>MGHHHHHHMLHLLEQIRAYCETCWEWQEAHEPGMDQDKNPMPAPVEHQICPAVCVLMKLSFDEEHRHAMNELGGLQAIAELLQVDCEMYGLTNDHYSITLRRYAGMALTNLTFGDVANKATLCSMKGCMRALVAQLKSESEDLQQVIASVLRNLSWRADVNSKKT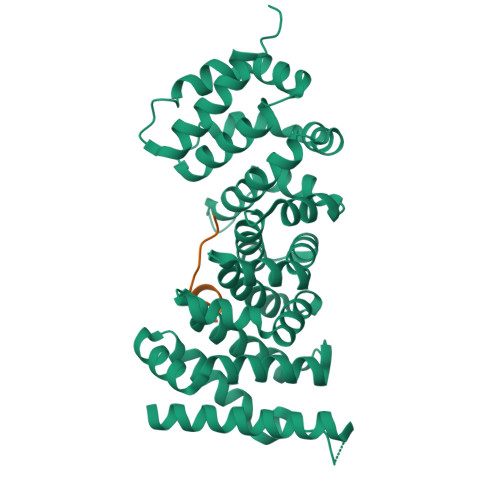LREVGSVKALMECALEVKKESTLKSVLSALWNLSAHCTENKADICAVDGALAFLVGTLTYRSQTNTLAIIESGGGILRNVSSLIATNEDHRQILRENNCLQTLLQHLKSHSLTIVSNACGTLWNLSARNPKDQEALWDMGAVSMLKNLIHSKHKMIAMGSAAALRNLMANRPAKYKDANIMSPGSSLPS[3x];>[3x]SSSHHYSHPGGGGEQLAINELISDG>[4x]MNLFYNKEAVGDVAFLQINPTEGEYNYVTQGDVVEIQNDGEVVGYNIFNASNKATLTGNGHIKLTETL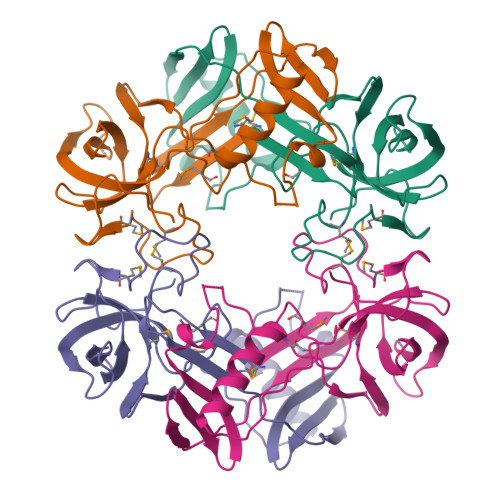VQAFQKAIEAAGFTYKLDADFTPKFVVGYVETKDKHPDADKLSVLSVDVATEKLQIVCGAPNVEAGQKVVVAKVGAVMPSGMVIKDAELRGVASSGMICSMKELGLPNAPQEKGIMVLSDDYTVGQSFFEV> MFRQCAKRYASSLPPNALKPAFGPPDKVAAQKFKESLMATEKHAKDTSNMWVKISVWVALPAIALTAVNTYFVEKEHAEHREHLKHVPDSEWPRDY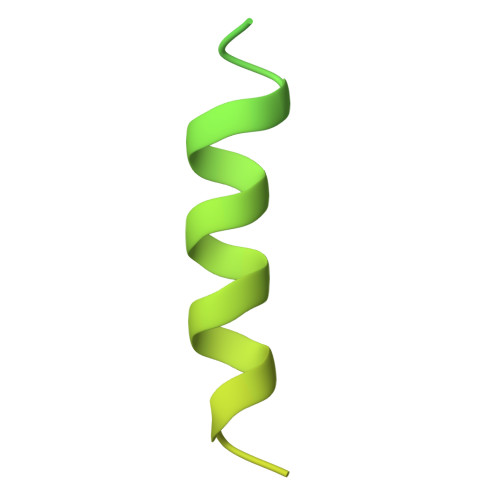EFMNIRSKPFFWGDGDKTLFWNPVVNRHIEHDD> GPEFPNDYDFMEDILDETMKSTFKSEYPFEKRKAESERIADRFPNRIPVICEKAEKSDIPEIDKRKYLVPADLTVGQFVYVIRKRIMLPPEKAIFIFVNDTLPPTAALMSAIYQEHKDKDGFLYVTYSGENTFG

Landmark proteins called autophagy receptors bind specific targets and interact with Atg8-family proteins on the isolation membrane through the Atg8-family-interacting motif (AIM) (also called the LC3-interacting region, LIR). The core of the AIM is composed of four amino-acid residues [W/F/Y]-X-X-[L/I/V]28. The first aromatic residue and the fourth aliphatic residue bind to two hydrophobic pockets in Atg8 (the W- and L-sites, respectively), and the main chain of the motif forms an intermolecular parallel β-sheet with a β-strand (β2) of Atg828. Nonetheless, deletion of the short helix from RTN3245–264 reduced the interactions with mAtg8s. Thus, the C-terminal helix-assisted AIM/LIR is a unique structural basis commonly seen in the interactions of yeast Atg40 and these mammalian ER-phagy receptors with Atg8-family proteins.

To elucidate the structural basis of the Atg40–Atg8 interaction, we determined the crystal structure of Atg8 N-terminally fused with the C-terminal sequence of Atg40 (Atg40237–252) containing the AIM (Y242-D-F-M). As with canonical AIMs, the first and fourth residues Y242 and M245 bound to the W- and L-sites of Atg8, respectively. In addition, the second residue D243 formed salt bridges with the R67 residue of Atg8. Moreover, the Atg40 region C-terminal to M245 assumed a helical conformation, and D247 in this helix formed salt bridges with R67 of Atg8. Residue F238 on the N-terminal side of the core motif also interacted with I21 and the aliphatic portion of R20 of Atg8. We prepared two “wild-type” peptides, Atg40234–252 and Atg40237–252, because the former peptide with the M245A and D243A D247A mutations could not be synthesized. Both Atg40234–252 and Atg40237–252 bound Atg8 with similar Kd values (0.59 ± 0.32 μM and 0.57 ± 0.51 μM, respectively). Importantly, ER-phagy was defective in cells expressing the D243A, D247A, and F238A mutants of Atg40, demonstrating that enhancement of Atg40 binding to Atg8 by these additional interactions is required for ER-phagy. Our structural analysis revealed that residue M245 bound properly to the L-site on Atg8; thus Atg40 is the first example of a protein in its class that uses methionine at the fourth position of the AIM. However, in Atg40, the main chain at M245 was included in the C-terminal helix, and thus distant from Atg8, enabling accommodation of methionine’s long side chain in the L-site.>MVLYFIGLGLYDERDITVKGLEIAKKCDYVFAEFYTSLMAGTTLGRIQKLIGKRIRVLSREDVELNFENIVLPLAKENDVAFLTPGDPLVATTHAELRIRAKRAGVESYVIHAPSIYSAVGITGLHIYKFGKSATVAYPEGNWFPTSYYDVIKENAERGLHTLLFLDIKAEKRMYMTANEAMELLLKVEDMKKGGVFTDDTLVVVLARAGSLNPTIRAGYVKDLIREDFGDPPHILIVPGKLHIVEAEYLVEIAGAPRE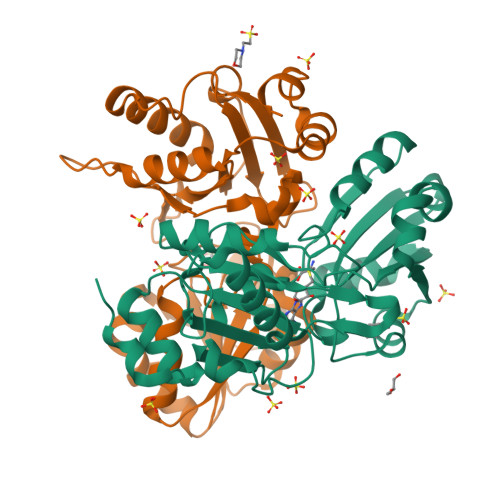ILRVNV[2x]(RP,SP)-O-(2R)-(1-PHENOXYBUT-2-YL)-METHYLPHOSPHONIC 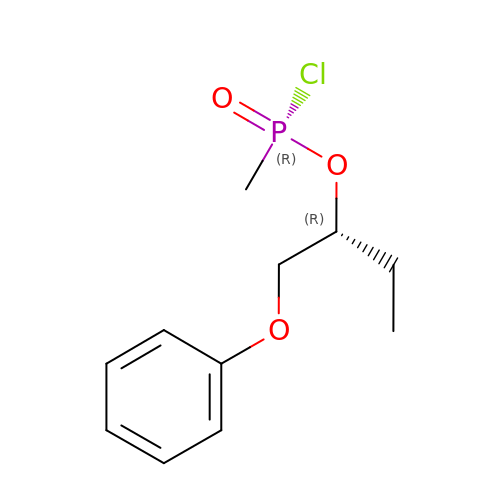ACID CHLORIDE | C11 H16 Cl O3 P | YEIXDWIEYXZUBR-QLJPJBMISA-N> MGAAYHFMGKAIPPHQLAI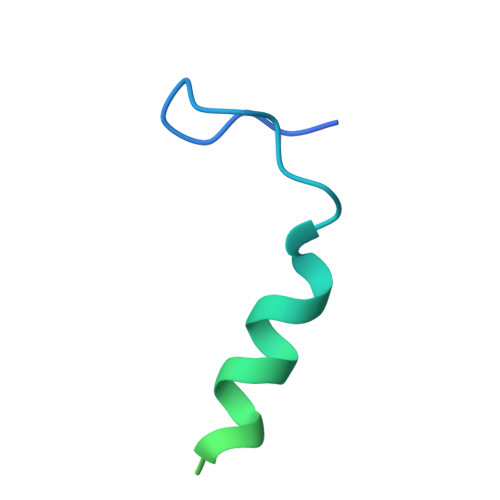GTLGLLGLLVVPNPFKSAKPKTVDIKTDNKDEEKFIENYLKKHSEKQDA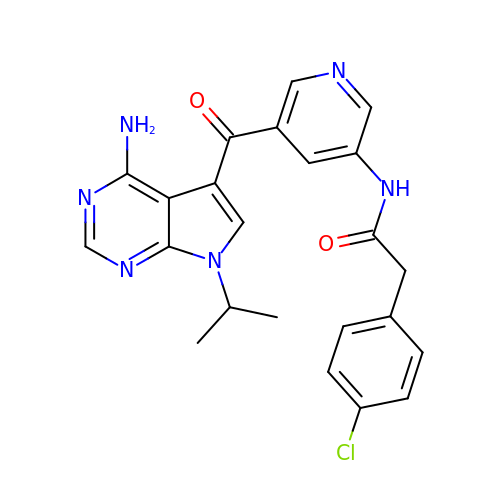N-{5-[4-amino-7-(propan-2-yl)-7H-pyrrolo[2,3-d]pyrimidine-5-carbonyl]pyridin-3-yl}-2-(4-chlorophenyl)acetamide | C23 H21 Cl N6 O2 | KVAUYQFSODRWMC-UHFFFAOYSA-N> GPLGSMEGFERELDNIPDTLPDDERLALWKGKLKHYLILSSAGKPIWSRHGDLSLVNSTMGVVQTIISFYEGARNPLLGFTAGKVRFVILIK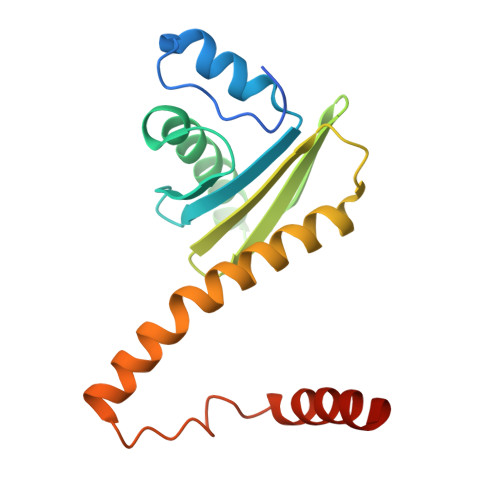GPLYFVAISRLRESDAQLRAQLEALYMQILSTLTLPILTNIFAHRPSTDLRGPLQGTESLLASLADSFTKGSPS> MSSGLYSMEKKEFDKVLDLERVKPYGDTMNDGKVQLSFTLPLKNNERSAEAAKQIALKMGLE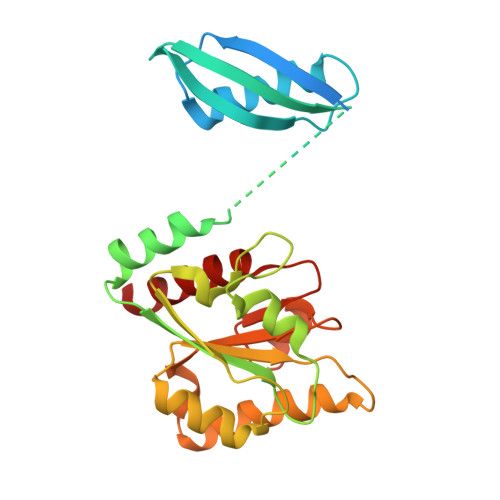EPSVVMQQSLDEEFTFFVVYGNFVQSVNYNEIHVEAVNSEILSMEETDEYIKENIGRKIVVVGASTGTDAHTVGIDAIMNMKGYAGHYGLERYEMIDAYNLGSQVANEDFIKKAVELEADVLLVSQTVTQKNVHIQNMTHLIELLEAEGLRDRFVLLCGGPRINNEIAKELGYDAGFGPGRFADDVATFAVKTLNDRMNS>[2x]MGSSHHHHHHGSGLVPRGSAGMAAPGENRRVNADRLWDSLMEMAKIGPGVAGGNNRQTLTDADGEGRRLFQSWCEEAGLSMGVDKMGTMFLTRPGTDPDALPVHIGSHLDTQPTGGKFDGVLGVLS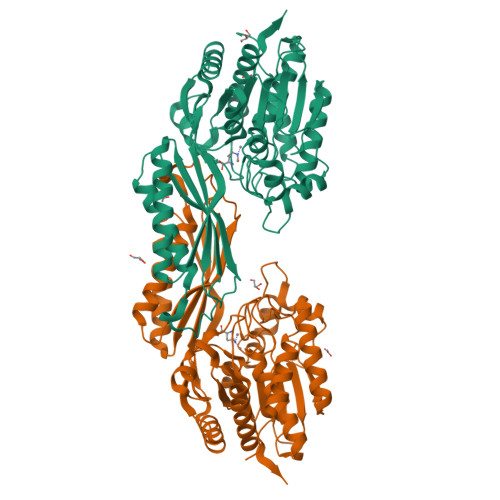GLEAVRTMNDLGIKTKHPIVVTNWTNEEGARFAPAMLASGVFAGVHTLEYAYARKDPEGKSFGDELKRIGWLGDEEVGARKMHAYFEYHIEQGPILEAENKQIGVVTHCQGLWWLEFTLTGREAHTGSTPMDMRVNAGLAMARILEMVQTVAMENQPGAVGGVGQMFFSPNSRNVLPGKVVFTVDIRSPDQAKLDGMRARIEAEAPKICERLGVGCSIEAVGHFDPVTFDPKLVETVRGAAEKLGYSHMNLVSGAGHDACWAAKVAPTTMIMCPCVGGLSHNEAEDISREWAAAGADVLFHAVLETAEIVE> FENGLGRTPQMGWNSWNHFYCGINEQIIRETADALVNTGLAKLGYQYVNIDDCWAEYSRDSQGNFVPNRQTFPSGIKALADYVHAKGLKLGIYSDAGSQTCSNKMPGSLDHEEQDVKTFASWGVDYLKYDNCNDAGRSVMERYTRMSNAMKTYGKNIFFSLCEWGKENPATWAGRMGNSWRTTGDIADNWGSMTSRADENDQWAAYAGPGGWNDPDMLEVGNGGMSEAEYRSHFSIWALAKAPLLIGCDVRSMSQQTKNILSNSEVIAVNQDSLGVQGKKVQSDNGLEVWAGPLSNNRK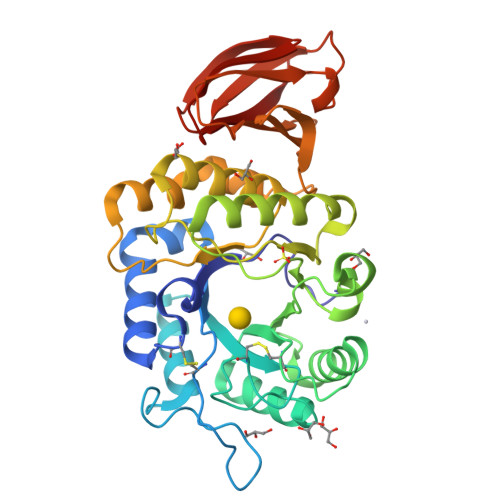AVVLWNRQSYQATITAHWSNIGLAGSVAVTARDLWAHSSFAAQGQISASVAPHDCKMYVLTPN>GAPDSWEAGVILIALGV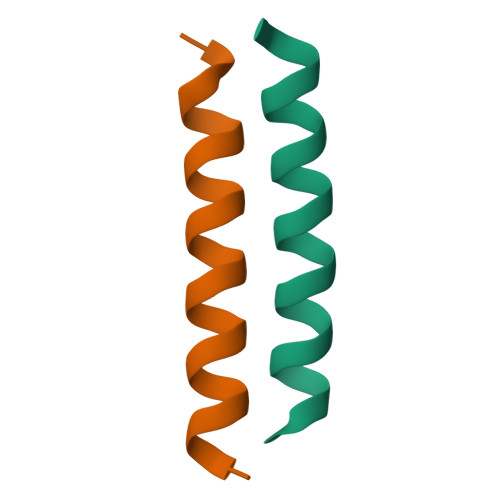FVLYLGVKLLKFA[6x]>ADTIVAVELDTYPNTDIGDPSYPHIGIDIKSVRSKKTAKWNMQDGKVGTAHIIYNSVDKRLSAVVSYPNADATSVSYDVDLNDVLPEWVRVGLSASTGLYKETNTILSWSFTSKLKSNSTHQTDALHFMFNQFSKDQKDLILQGDATTGTDGNLELTRVSSNGSPEGSSVGRALFYAPVHIWESSAATVSFEATFAFLIKSPDSHPADGIAFFISN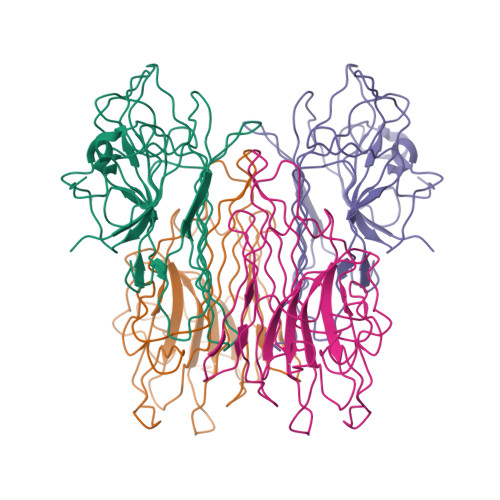IDSSIPSGSTGRLLGLFPDAN[2x]> APAFRYTRSQSFDIFDINQKCFVLESPTQLVALHLQGPSSSQKVRLNIALYRPRGPRGSAGTGQMPVALGIKGYKLYMSCVMSGTEPTLQLEEADVMRDIDSVELTRFIFYRLDSPTEGTTRFESAAFPGWFICTSLQPRQ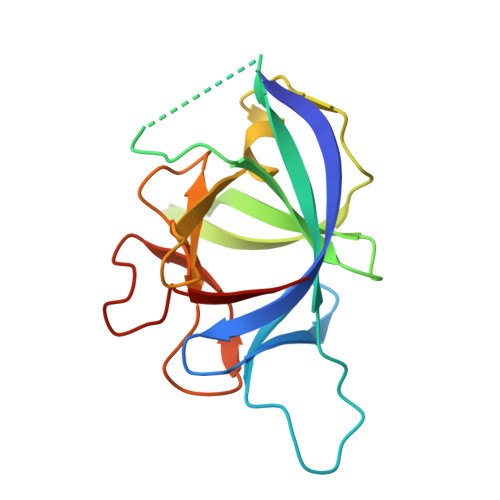PVGITNQPDQVNIATYKLSGR> MIKLRMPAGGERYIDGKSVYKLYLMIKQHMNGKYDVIKYNWCMRVSDAAYQKRRD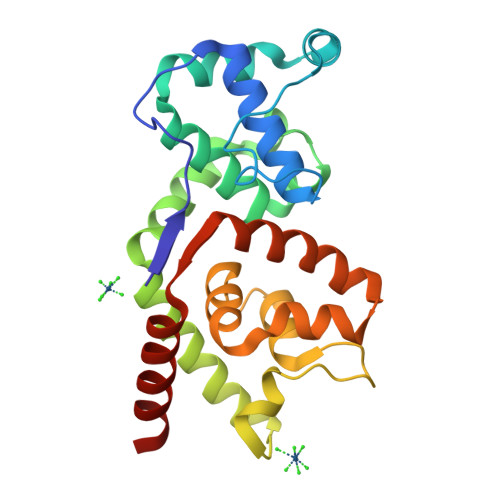KYFFQKLSEKYKLKELALIFISNLVANQDAWIGDISDADALVFYREYIGRLKQIKFKFEEDIRNIYYFSKKVEVSAFKEIFEYNPKVQSSYIFKLLQSNIISFETFILLDSFLNIIDKHDEQTDNLVWNNYSIKLKAYRKILNIDSQKAKNVFIETVKSCKY>[2x]MNDSE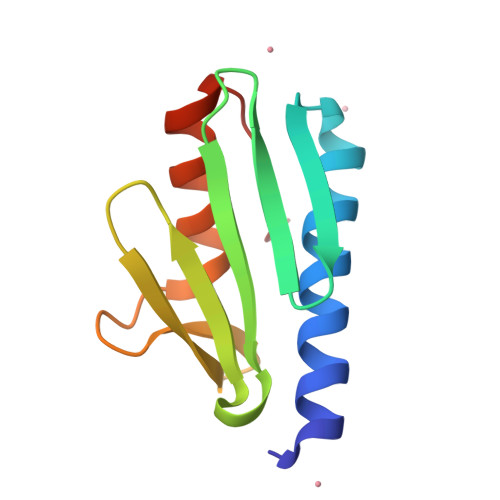FIQLADQLYQKIEEKIEESGADVDYDQNGSLLTLEFENHTKLIINRQQPLHQVWLATLENGHHYDYNNGKWIDDRSGDEFLTFLSAAIFKQSKETVDFTE>SGSWQTYVDEHLMCDIEGTGQHLASAAIFGTDGNVWAKSSSFPEFKPDEINAIIKEFSEPGALAPTGLFLAGAKYMVIQGEPGAVIRGKKGAGGIC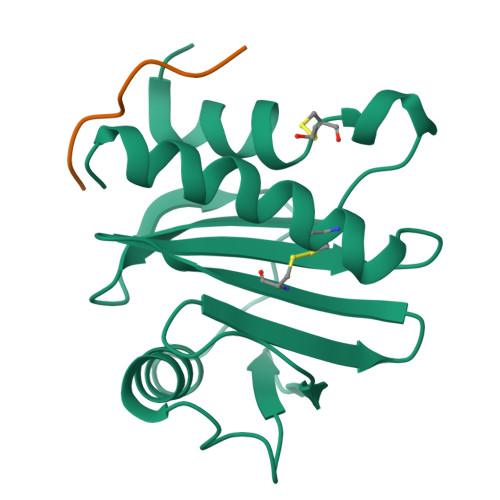IKKTGQAMVFGIYEEPVNPGQCNMVVERLGDYLVDQGM[2x];>PPPPPPPPP[2x]> MNKIN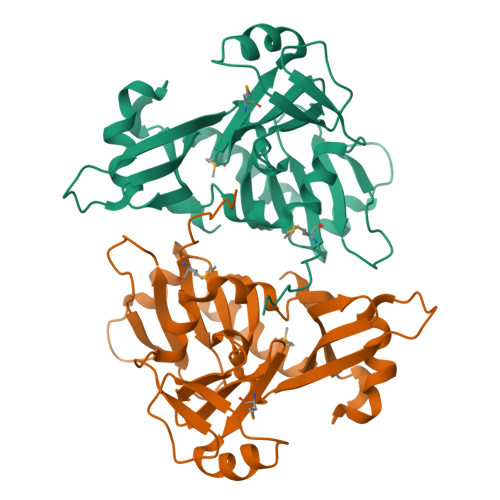ASPQAMLIVRLAAAQAPLHWQLFAPGEPHHEASGRWPTDDASPFPALAEQYPAWVLIPASDCAFHSLTLPAGLRKPPLQVAPFLLEEQLADDVEATHFALLHRQQAQCEIVAVQRQKMRDWLARCESLSLQPLALTPDVLALPWQPPAWSAVQVDEQWLIRHQPWGGMAAENVWLTELLQSEAEEHVIDSYSPPPAAPGVWREQPAQTLLTLAARHPAAQKLSLLQGEFAVR(5R)-2-amino-5-(4-fluoro-3-pyrimidin-5-ylphenyl)-3-methyl-5-[4-(trifluoromethoxy)phenyl]-3,5-dihydro-4H-imidazol-4-one 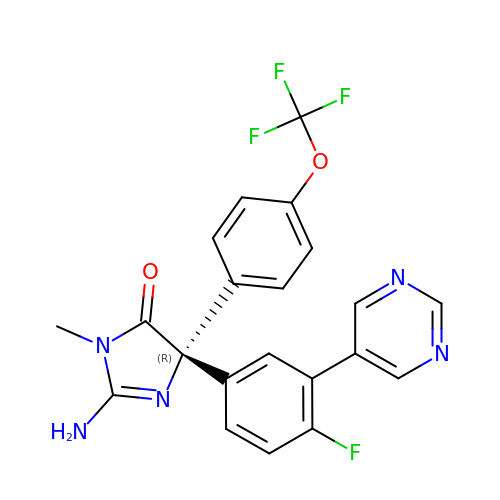| C21 H15 F4 N5 O2 | RNJTYVPMRSKRKE-HXUWFJFHSA-N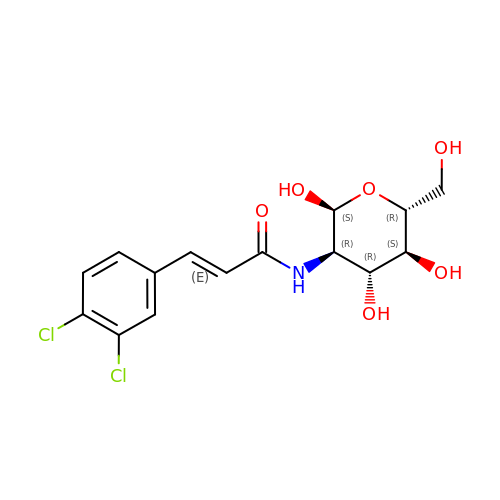2-deoxy-2-{[(2E)-3-(3,4-dichlorophenyl)prop-2-enoyl]amino}-alpha-D-glucopyranose | C15 H17 Cl2 N O6 | ZBHWRKZTEDNOAJ-GJAUZLMESA-N> AASDWKPGYSMPVLYKYLNSPMERVSLWNYGKPVTLPTGCMMNVAKYTQLCQYLNTTTLAVPVNMRVLHLGAGSEKGVAPGSAVLRQWLPAGTILVDNDLYPFVSDSVATYFGDCITLPFDCQWDLIISDMYDPITKNIGEYNVSKDGFFTYICHMIRDKLALGGSVAIKITEFSWNAELYKLMGYFAFWTVFCTNANASSSEGFLIGINYLCKPKVEIDGNVMHANYLFWRNSTVWNGGAYSLFDMAKFPLKLAGTAVINLRADQINDMVYSLLEKGKLLIRDTNKEVFVGDSLVNVI;> NSSILSLCAFSVDPKKTYLDFIQQGGTPIANCVKMLCDHAGTGMAITVKPDATTSQDSYGGASVCIYCRARVEHPDVDGLCKLRGKFVQVPVGIKDPVSYVLTHDVCRVCGFW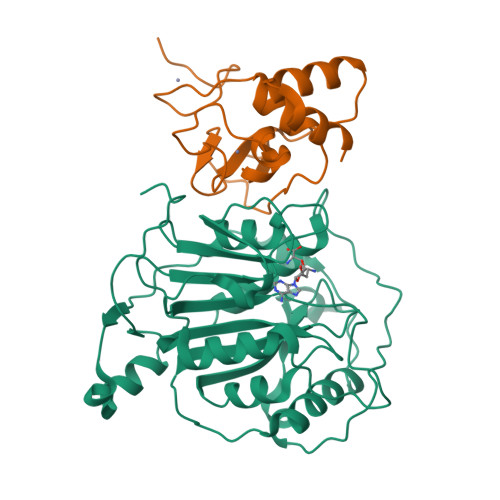RDGSCSCVS> MRVLGIETSCDETGIAIYDDEKGLLANQLYSQVKLHADYGGVVPELASRDHVRKTVPLIQAALKESGLTAKDIDAVAYTAGPGLEGALLVGATVGRSLAFAWDVPAIPVHHMEGHLLAPMLEDNPPEFPFVALLVSGGHTQLISVTGIGQYEL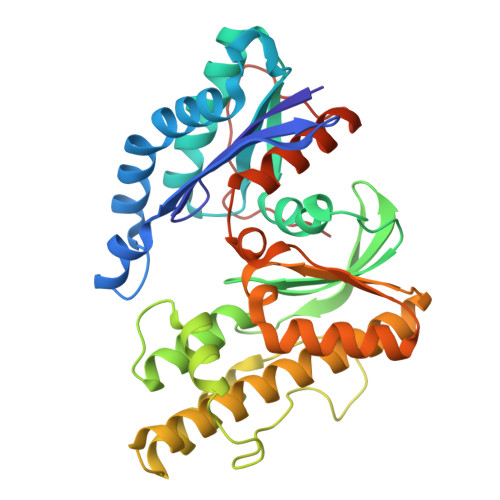LGESIDDAAGEAFDKTAKLLGLDYPGGPLLSKMAAQGTAGRFVFPRPMTDRPGLDFSFSGLKTFAANTIRDNGTDDQTRADIARAFEDAVVDTLMIKCKRALDQTGFKRLVMAGGVSANRTLRAKLAEMMKKRRGEVFYARPEFCTDNGAMIAYAGMVRFKAGATADLGVSVRPRWPLAELPAAHHHHHH> AGRFTKVAAAVADSVVTIESVSDQEGMQGSGVIVDGRGYIVTNNHVISEAANNPSQFKTTVVFNDGKEVPANLVGRDPKTDLAVLKVDNVDNLTVARLGDSSKVRVGDEVLAVGAPLGLRSTVTQGIVSALHRPVPLSGEGSDTDTVIDAIQTDASIAHGNSGGPLIDMDAQVIGINTAGKSLSDSASGLGFAIPVNEMKLVANSLIKDGKIVHPTLGISTRSVSNAIASGAQVA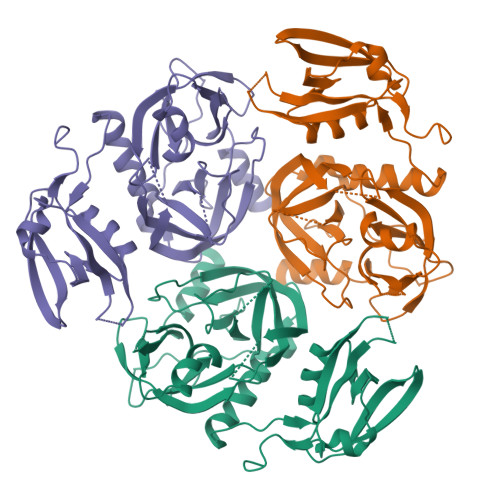NVKAGSPAQKGGILENDVIVKVGNRAVADSDEFVVAVRQLAIGQDAPIEVVREGRHVTLTVKPDPDSTLEH> MGHMNITDIREQFPILHQQVNGHDLVYLDSAATSQKPRAVIETLDKYYNQYNSNVHRGVHTLGTRATDGYEGAREKVRKFINAKSMAEIIFTKGTTTSLNMVALSYARANLKPGDEVVITYMEHHANIIPWQQAVKATGATLKYIPLQEDGTISLEDVRETVTSNTKIVAVSHVSNVLGTVNPIKEMAKIAHDNGAVIVVDGAQSTPHMKIDVQDLDCDF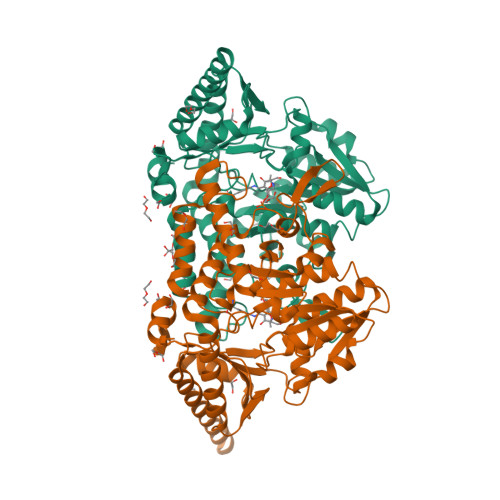FALSSHKMCGPTGVGVLYGKKALLENMEPAEFGGEMIDFVGLYESTWKELPWKFEAGTPIIAGAIGLGAAIDFLEEIGLDEISRHEHKLAAYALERFRQLDGVTVYGPEERAGLVTFNLDDVHPHDVATVLDAEGIAVRAGHHAAQPLMKWLDVTATARASFYLYNTEEEIDKLVEALQKTKEYFTNVFVDLEHHHHHH>MRGSHHHHHHR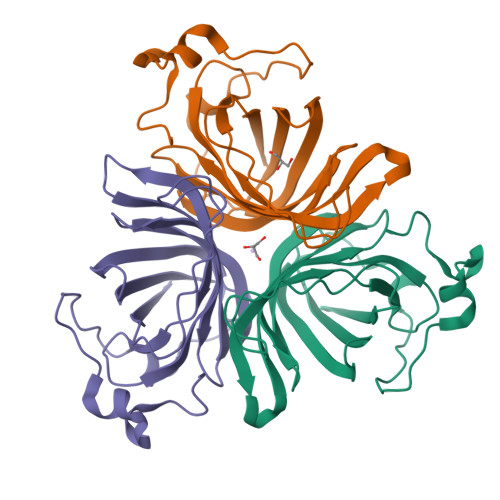SPSKVQELSVYEINELDRHSPKILKNAFSLMFGLGDLVPFTNKLYTGDLKKRVGITAGLCVVIEHVPEKKGERFEATYSFYFGDYGHLSVQGPYLTYEDSFLAITGGAGIFEGAYGQVKLQQLVYPTKLFYTFYLKGLANDLPLELTGTPVPPSKDIEPAPEAKALEPSGVISNYTN[6x]The most abundant virulence factor secreted by Hc yeast cells is Calcium Binding Protein 1 (Cbp1), which is absolutely required for macrophage lysis. The mature secreted form of Cbp1 is 78 amino acids in length, has no known domains, and, prior to this work, had only one known homolog in the closely related fungus Paracoccidioides. The Cbp1 structures displayed an alpha-helical dimer arrangement with an intermolecular four-helix bundle fold at the core formed from the 3rd and 4th helices of each monomer, creating a binocular shape, and thus we dubbed this new arrangement as a “binocular” fold. For both Pb03 and H88 Cbp1, the three disulfide bonds present in each monomer orient the alpha helices so that the aromatic residues (Phe12, Phe19, Trp30) are packed in the interior of the protein, creating the hydrophobic core.

Additionally, we have previously shown that the Paracoccidioides americana (Pb03) homolog of Cbp1 is capable of fully restoring lytic capability when expressed in a Hc cbp1 mutant background, suggesting that Hc is not the only species that could be using Cbp1 to elicit host cell death. Mass spectrometric analysis of Pb03 Cbp1 revealed two signal sequence cleavage sites, which likely explain the doublet on SDS-PAGE. Crystals of Hc H88 and Pb03 Cbp1 homologs formed after a week and diffracted to 1.6 Å. To resolve the phases, a heavy atom derivative was prepared by soaking the Pb03 crystals in K2PtCl4. The structure of Pb03 was truncated at C-terminal residues 65–67 from chain A and 67–68 from chain B, as the remaining amino acids were not resolved in the refined density. The asymmetric unit for the Pb03 Cbp1 crystal contained a single dimer, whereas the asymmetric unit for the H88 crystal contained a dimer of dimers. An alignment of the Pb03 and the Hc CBP1 dimers gave an RMSD of 1.6 Å, indicating the structures of the distinct homologs are conserved. The Pb03 structure has a clear negative charge at the C-terminal end of the protein and was partially positive at the interface between the N-terminal helices. Interestingly, only the Pb03 (and not H88) structure shows partially negative N-terminal helices. Using a N-terminal FLAG-tagged Pb03 Cbp1 homolog that retains its lytic capability during infection, we confirmed the cytosolic localization of Pb03 Cbp1 via this subcellular fractionation approach.

>[2x]AQPAVKHALGQFNQVVTMFEKATAAASCNWITCLESLAASSAACAAALGELGLDIPLDLACIASAASTSAQGCEGCF There are three parts to the flagellar structure: the trans-membrane basal body that functions as the motor, the connecting rod and hook, and the flagellar filament that acts like a helical propeller. Our current understanding of supercoiling in bacterial flagellar filaments, referred to as polymorphic switching, is based upon the notion that protofilaments within the flagellar filament can exist in two discrete states, that differ slightly in length. The “short” state results from a protofilament having a right-handed inclination (the R-state), while the “long” state results from a protofilament having a left-handed inclination (the L-state). To reconstruct filaments at high resolution, all protofilaments must be “locked” into the same state, either L- or R-type, producing straightened filaments that lead to non-motile bacteria.

We also included a previously identified straight filament mutant, HagA233V, in the study. While the three L-type mutants (E115G, S285P, and S17P) have a left-handed 11-start helix, the four R-type mutants (N226Y, A233V, H84R and A39VN133H) have a right-handed 11-start helix, and the designations L and R correspond to the hand of these 11-start helices. The L-type 11-start helices are tilted left by ~ 1.7° and the R-type 11-start helices are tilted right by ~ 3.9°. Another example is the R-type mutant A233V in B. subtilis. A233 is conserved among Gram-positive species but not in Gram-negative species. In the A233V mutant, valine in subunit S0 makes stronger contacts than an alanine residue with the hydrophobic pockets formed by A43, L46 and A47 in subunit S+11, and A233V filaments adopt a right-handed form.

>MRINHNIAALNTLNRLSSNNSASQKNMEKLSSGLRINRAGDDAAGLAISEKMRGQIRGLEMASKNSQDGISLIQTAEGALTETHAILQRVRELVVQAGNTGTQDKATDLQSIQDEISALTDEIDGISNRTEFNGKKLLDGTYKVDTATPANQKNLVFQIGANATQQISVNIEDMGADALGIKEADGSIAALHSVNDLDVTKFADNAADCADIGFDAQLKVVDEAINQVSSQRVKLGAVQNRLEHTINNLSASGENLTAAESRIRDVDMAKEMSEFTKNNILSQASQAMLAQANQQPQNVLQLLR[46x]>MVGSLNCIVAVSQNMGIGKNGDLPWPPLRNEFRYFQRMTTTSSVEGKQNLVIMGKKTWFSIPEKNRPLKGRINLVLSRELKEPPQGAHFLSRSLDDALKLTEQPELANKVDMVWIVGGSSVYKEAMNHPGHLKLFVTRIMQDFESDTFFPEIDLEKYK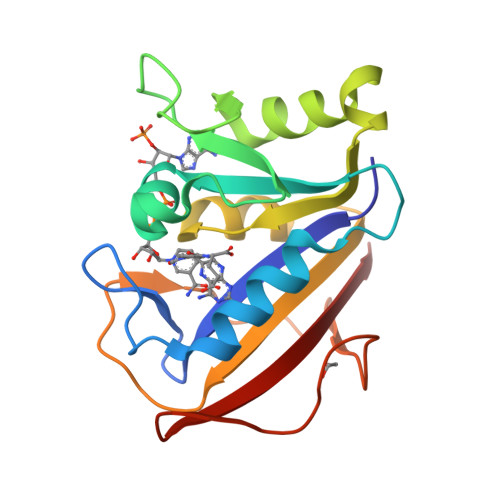LLPEYPGVLSDVQEEKGIKYKFEVYEKND[2x]>[6x]MADKAKPAKAANRTPPKSPGDPSKDRAAKRLSLESEGAGEG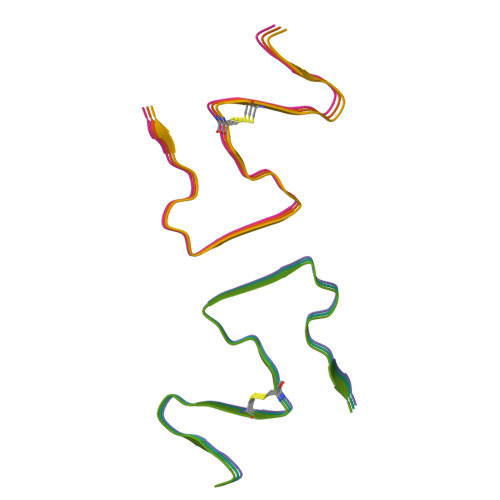AAASPELSALEEAFRRFAVHGDARATGREMHGKNWSKLCKDCQVIDGRNVTVTDVDIVFSKIKGKSCRTITFEQFQEVLEELAKKRFKDKSSEEAVREVHRLIEGKAPIISGVTKAISSPTVSRLTDTTKFTGSHKERFDPSGKGKGKAGRVDLVDESGYVSGYKHAGTYDQKVQGGK>DCNILQRLKVKMQWAKAYGFGTERAKFGNSLWTSIFNYAPDARDLFKSVKSEDMRSPQFKAHIARVIGGLDRVISMFDNEDALNADLEHLKSQHDPRGLDALNFVVFGKALFATVGGQFGVCFDLPAWESCYKVIAMGITGNDMFS[2x];>[2x]SECGPLQRLKVKRQWAEAYGSGNGREEFGHFIWANVFKVAPSARDMFKRVRGDNIYTPAFRAHATRVLGGLDMCVALLDDESVLNTQLAHLASQHSSRGVSAEQYNVVEHAVMMGVEHEIGQNVFDKDAWQACLDVITSGIQGN;>[2x]SSNSCTTEDRREMQLMWANVWSAQFTGRRLAIAQAVFKDLFAHVPDAVGLFDRVHGTEIDSSEFKAHCIRVVNGLDSAIGLLSDPSTLNEQLSHLATQHQERAGVTKGGFSAIAQSFLRVMPQVASCFNPDAWSRCFNRITNGMTEGLAE;>[2x]SEFCSEADATIVIKQWNQIYNAGIGAKSRWTMGNEIFSSLFKLKPESEVLFNNVNVANMSSGAFHAHTVRVLSGLDMGINYLNDAGTLTSLT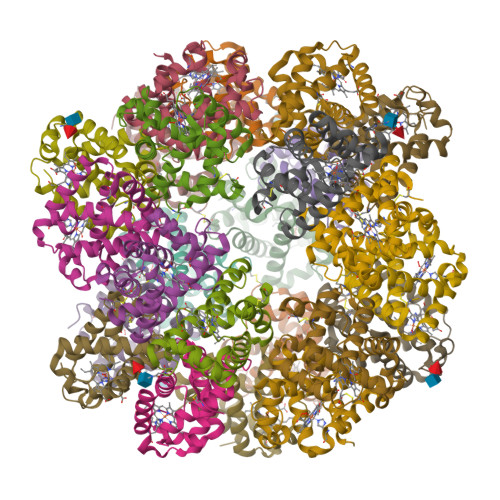AHLAAQHVARTGLKAVYFDAMGKVLMTVLPSLIDNFNPDAWRNCLLPLKNAIAKGLP>[2x]ADFEVH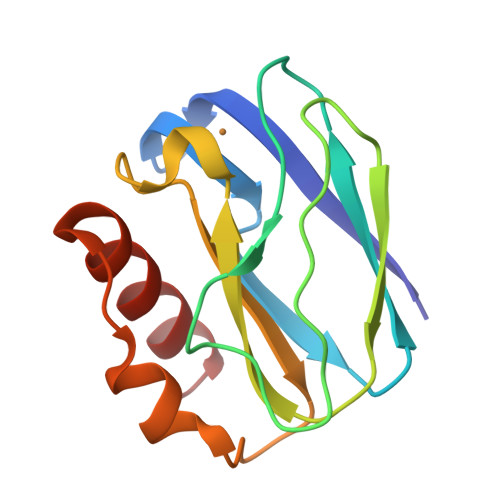MLNKGKDGAVVFEPASLKVAPGDTVTFIPTDKGHNVETIKGMIPDGAEAFKSKINENYKVTFTAPGVYGVKCTPHYGMGMVGVVQVGDAPANLEAVKGAKNPKKAQERLDAALAALGN Exo-β-mannosidases, hydrolysing non-reducing terminal β-d-mannopyranosidic linkages, are widely distributed carbohydrate-degrading enzymes. All of these exo-β-mannosidases process their substrate using a stereochemically retaining double displacement mechanism that is characterised by the formation of a covalent glycosyl enzyme intermediate (GEI). We show that these probes covalently label exo-β-mannosidases from GH families 2, 5, and 164. Structural studies of the resulting complexes support a canonical mechanism-based mode of action in which the active site nucleophile attacks the pseudoanomeric centre to form a stable ester linkage, mimicking the glycosyl enzyme intermediate.

To test this hypothesis, we performed an extensive soak (10 mM, 4 days) of BtMan2A crystals with compound 2. Surprisingly, the resulting electron density map showed similar diffusion of electron density and rearrangement of the active site, with the ligand observed further displaced from the expected GEI in a highly unusual 1C4-like ring conformation in molecule A (ESI Fig. 2B†). In molecule B the ligand is 4C1-like (similar to the complex with the alkyl aziridine 3) and part unreacted aziridine (at occupancies 0.4 and 0.6 respectively). We thus conclude that there exists a more fundamental instability in the GEI structure of BtMan2A, possibly explaining earlier failures to trap it.

>[2x]MGQGNDTSEVMLLDTGWEFSQSGTEKWMPATVPGTVHQDLISHELLPNPFYGMNEKKIQWVENEDWEYRTSFIVSEEQLNRDGIQLIFEGLDTYADVYLNGSLLLKADNMFVGYTLPVKSVLRKGENHLYIYFHSPIRQTLPQYASNGFNYPADNDHHEKHLSVFSRKAPYSYGWDWGIRMVTSGVWRPVTLRFYDIATISDYYVRQLSLTDENARLSNELIVNQIVPQKIPAEVRVNVSLNGTTVTEVKQQVTLQPGINHITLPAEVTNPVRWMPNGWGTPTLYDFSAQIACGDRIVAEQSHRIGLRTIRVVNEKDKDGESFYFEVNGIPMFAKGANYIPQDALLPNVTTERYQTLFRDMKEANMNMVRIWGGGTYENNLFYDLADENGILVWQDFMFACTPYPSDPTFLKRVEAEAVYNIRRLRNHASLAMWCGNNEILEALKYWGFEKKFTPEVYQGLMHGYDKLFRELLPSTVKEFDSDRFYVHSSPYLANWGRPESWGTGDSHNWGVWYGKKPFESLDTDLPRFMSEFGFQSFPEMKTIAAFAAPEDYQIESEVMNAHQKSSIGNSLIRTYMERDYIIPESFEDFVYVGLVLQGQGMRHGLEAHRRNRPYCMGTLYWQLNDSWPVVSWSSIDYYGNWKALHYQAKRAFAPVLINPIQQNDSLSVYLISDRLDTMEQMTLEMKVVDFDGKTLGKKIQVHSLEVPANTSKCVYRAKLDGWLTPEDCRRSFLKLILKDKSGHQVAESVHFFRKTKDLQLPPTSVSYQMKQTDGKCELTLFSSMLAKDIFIETPLQGARYSDNFFDLLPGERKKVIITSPRIKKGEELPVNIKHIRETYKLEHHHHHH> AAPAYGQPSAAMGQNMRPMNQLYPIDLLTELPPPITDLTLPPPPLVIPPERMLVPSELSNASPDYIRSTLNAVPKNSSLLKKSKLPFGLVIRPYQHLYDDIDPPPLNEDGLIVRCRRCRSYMNPFVTFIEQGRRWRCNFCRLANDVPMQMDQSDPNDPKSRYDRNEIKCAVMEYMAPKEYTLRQPPPATYCFLIDVSQSSIKSGLLATTINTLLQNLDSIPNHDERTRISILCVDNAIHYFKIPLDSENNEESADQINMMDIADLEEPFLPRPNSMVVSLKACRQNIETLLTKIPQIFQSNLITNFALGPALKSAYHLIGGVGGKIIVVSGTLPNLGIGKLQRRNESGVVNTSKETAQLLSC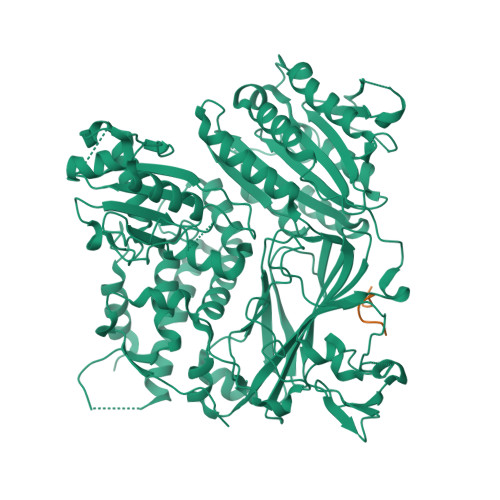QDSFYKNFTIDCSKVQITVDLFLASEDYMDVASLSNLSRFTAGQTHFYPGFSGKNPNDIVKFSTEFAKHISMDFCMETVMRARGSTGLRMSRFYGHFFNRSSDLCAFSTMPRDQSYLFEVNVDESIMADYCYVQVAVLLSLNNSQRRIRIITLAMPTTESLAEVYASADQLAIASFYNSKAVEKALNSSLDDARVLINKSVQDILATYKKEIVVSNTAGGAPLRLCANLRMFPLLMHSLTKHMAFRSGIVPSDHRASALNNLESLPLKYLIKNIYPDVYSLHDMADEAGLPVQTEDGEATGTIVLPQPINATSSLFERYGLYLIDNGNELFLWMGGDAVPALVFDVFGTQDIFDIPIGKQEIPVVENSEFNQRVRNIINQLRNHDDVITYQSLYIVRGASLSEPVNHASAREVATLRLWASSTLVEDKILNNESYREFLQIMKARISK;> QLKDLESQI> PNIEMFVVEGYSDQQKEALVGALTQATVEAIGAPIDSVRVWLTEVPATQFGIGGKT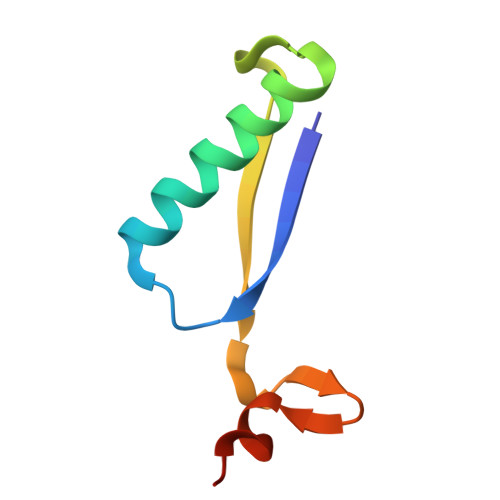VAAIAAGQE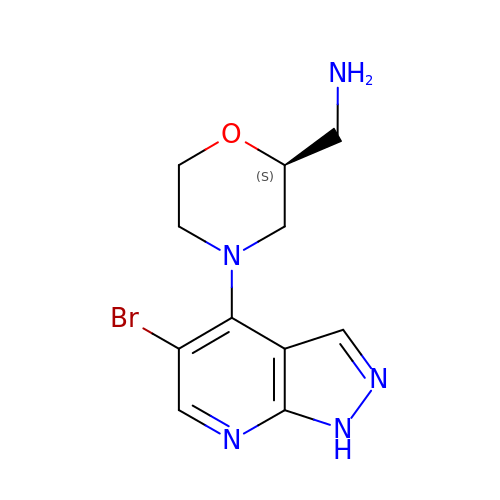1-[(2S)-4-(5-BROMO-1H-PYRAZOLO[3,4-B]PYRIDIN-4-YL)MORPHOLIN-2-YL]METHANAMINE | C11 H14 Br N5 O | BJUBFXSKTBULRW-ZETCQYMHSA-N>MQALRRGAAIPSRLLPRRDSWMSLAPFVAPNNAAAWRKLRDGAQEVQTVIERQSTPGKPQQIDWAKWESQIAHKDILNCLKTFYTNQVQILDRALGALETAKTPAPCEGAEKGWALFDAALSACAKSVEKSEELLSNGARALWVSCSNPPVWKVNTNEWLDSDQYWQAFVEKHHFYSQYQPGVVDPEAPQEVEAFKQAWHSRMGKFNDRSDTPMLYAYMNELPSWEYYDLHRSAFLEHMTYFLVRTGGDFRFFPEMPPWQWLAHMENLRFKLLSVAQSRRSQLQLANLERERALDFLPVDVEHHGEEYTQKFLQYETELFQACAARLMGHFMFLCDPFIPVQSAEALSAVTRVDNGKGKLFSLGDDVNALFYLPEQQRRDVERPTQAVQTLLGHLEATGRPFNPCYSELLHVHAEVLEERGEHWLTAPGECVSQAFLRRLRTDDPAYEVYCSYFKEMYERFAGAKEVSMEDGRKRLATIEKNAQEEAAAYGLALKTMGSAELAHKAREGAAKLEQLRKAQEKAAGKSAQTVQENKM[2x];>MTIHSCLARRAVSVAASGARAFASGLGARAVAVGALQSARLLHTSSLRAAGAKISPSEMSRLLEERIAGWKTQTSTEEVGRVVSVGDGIARLFGLEGVQAGELVEFQNGMTGMALNLETDNVGVVIFGDDRSVLEGDSVKRTGRIVDVPIGPGLLGRVVDALGNPIDGKGPIPAKERRRVELKAPGIIPRKSVHEPMMTGLKCVDALVPVGRGQRELIIGDRQTGKTAVAVDAIINQKEINDSTDDESKKLYCIYVAVGQKRSTVAQIVKALEQRDAMKYTTVVAATASEAAPLQFLAPYSGCAMGEWFRDSGRHCVIIYDDLSKQATAYRQMSLLLRRPPGREAYPGDVFYLHSRLLERAAKMGDKSGGGSLTALPVIETQAGDVSAYIPTNVISITDGQIFLETELFYKGIRPAINVGLSVSRVGSAAQVKAMKQVAGTMKLELAQYREVAAFAQFGSDLDASTRQLLTRGTALTELLKQRQYSPMKNSVQVCVLYCGVKGYLDPLDPKEISRFESLFIDYINANHQDILKTIETEKELSEKTEAKLRAAVDEFVAMNEFKKK[6x];>[2x]MNFSSSARWLAVRQSQTLGHTTRATVAAGRRVLAHSPAATEFTSFQSLHIGGDVCKLPLAVALGAAPSALGYGSAKHNQQRQYATLGSGWSFSKVQYTKYRITKPWTTDTTFDDIILSQPSKEDFAKFTKEAPLFLRFLKLVTDVEGRQEAFIQFAKRCENGLTVEKDVYVTKKELVDCLWKNGYTDTEINAFEIAFPADYKFHYPELAVLFDLTEEDCYKYCIRQRAATPEELVELKYTKPKNLVSSYGLCFLGVWFGLSNTVLSNAWFYSKTFPFGAVFYMLGSYFYRDIREKLWKEEKSLIHTAQENKNMGEESVYKQMKKYATDTKCLDYLSTFRTEVEDQIANYKVALVSQMRRQLTERLVEKLNGIQQAEKLIQGSLQDVMIREIVSSFKDLYKSRPELHDAAMQSAIQGLSGSDGAMDPVGAHFKASLQELAKVNLSTATADPMGTVVQRVAAVFQKREKEFLDTFTVKATEAQEIKTIVDKCHKGNTFDFHALSDEELRRLEQLYSTVNNRVGFETIHENSIKPVAPLSENSKGFVEFVNTQLEITKAKLRNARLTAFAHAFV;>[6x]MASPALQTCWRNLARLSGAQVRPSHFGAFSLGSRMSPFSSLLGARASPIATGRAGLRFLSSAAPNPGKKPASAAPPAGTNHGRITQVIGAVVDVHFDEQLPPILNSLEVQGHTNRLVLEVAQHLGENTVRTIAMDATEGLVRGQKVVDTGAPIQVPVGVETLGRIMNVIGEPVDECGPVPAKKTYSIHRAAPLFADQSTEPGLLQTGIKVVDLLAPYAKGGKIGLFGGAGVGKTVLIMELINNVANKHGGFSVFAGVGERTREGNDLYHEMMTTGVIKRKKLEDGKFDFTGSKAALVYGQMNEPPGARARVALTALSVAEYFRDEQGQDVLLFIDNIYRFTQAGSEVSALLGRIPSAVGYQPTLATDLGQLQERITTTKKGSITSVQAVYVPADDLTDPAPATTFAHLDATTVLSRQIAELGIYPAVDPLDSTSRMLAPEIVGQEHYDTARATQKLLQDYKSLQDIIAILGMDELSEEDKLVVSRARKIQRFLSQPFTVAEVFTGKPGRFVELPETIKSAQTILRGECDDLPEMAFYMCGGLEEVRSKAVKMAQEAASGK;>MGGGGGGALNKLFPGYKDKIWMKVPVQWRQQMIQHWNKSYEKQVYSESVALNRTFQARNQLVLDRLKPSGAYRLPAVDYKRQLSRGTLVEGADFYLPTAQEQQRLARHFEPYSEQEQEERRKFRFQSISVYLAVALGASFVHDYFYQRRPVAWCLEKEPPHPPSYPFWFKSLFHSHDIPSVRRGYEVYRKVCATCHSMEQLHFRHLVGEVLPEKRVKQIAAEYDVTDGPNDQGEMYTRPGILGDAFPSPYPNEEAARYANGGAYPPDLSLITAARHFGPDYLMALLGGYRDPPEGVELRPGLYWNVWFPGNAIAMPPPLMDEMIDYEDGTPCNISQMSKDVVNFLTWATEPTADERKLYGLKCVSAIAIGTVLMTLWWRFYWAMYATRRIDFGKLKYL[2x];>MSPVGRLFLGSKLPAQTWQSFRLQPALPQFAQKRFFSGGAAKPSWHVAREHRFGPTLPDHAYYGEHATYNYFVLFIRGMRPYLEKIFGDCASTIKNAAVAVYRPVNAFVVKHNPDLRLQFVAFASFIATHMAITKEFNDMYQRLVDITSLLELQAAQLHASEGFWDSESEQQEARLQRHAEHRNDLETTWEEALREATLARNFDVLVSYLNHGTSDGCGEHGACGHSGQNGIPPSVTWNFNAMPYGKENPDTKTFPIPDHEQPYRAFSLGFTANNLSGNWGDYIDRQDNKNALMRPARMMFTDVFIPTTK[2x];>MGEKQEEEGEEEKEGKGEGGGEGGREEEDEDGSAPVVSWLRIVEERECHEETDEAPETKIALPFSAQRSSRGFEARQVEVLVSANSAFLLSVLLASLFLSSSLPSFCPPRFLLSVLLALFKDKMAGDAPAAAAAPQQAGRTASASGVRTPGYLDLVGHSLKATSMDHGMQYSSIYWETSHRTYLPFWASLTQKFSWKIMDDQIRSFLRLPKPVTTEPFVFSSGSPYIRRYFGDADISVPVPLHAPAHFAFVPTGTVSPWEETGMETGPQGAAARGAAATAFRAVLESAWKCDIDEQIKEKLHSRAGAGAFHASGSTGGCPIPTDF[2x];>MALNRVPSRVLPFAVSGVYVHPRNACRLPAAAAVSSVPSSVSAFSSRTNFLSRSSSAVMSHPCAATARHFSFAIPPANAAALADPLPATPTPPPVFEAVSSASSGIASGTNALKNVEEVSTMERYEAAVYEESFKKPIVCLFFARFSLQSKVLLQPFLDFAASASNNATFFLIDCDRVPRAAYHARVENVPSLVVMKGDDAFRQTITDSVGVKTAGDLIQEARSALDQVLRLDQQEGGTKLQPGVSSYTHHIGVDNLNVYRKGWPVA[2x];>[2x]MQNGVFTRENADFLVKSGADSPSSQSLLLRTSPSPLSLPRRRFIFLRSASVDLSERSSLACLAPFFCLASGVCLRSAFSLPFFARRGRPCLFFIFIFFFRVSFTANFRGKRVKMAASTIPISQWPSLLYAPPSSPANPAVEALPEMQFDDLHYPRQMLLCRGAGYSLEQCNRMAQPDARVTPENPAEKLLKEEAVAAIACLSQREGGKDEQCRYYIERMYKLANKEKQPEPGTLSKASTLACKLLGIHRPEA;>[2x]MALPLLASRRLFSSFVFRGQPSTLSSNLSLVRIRGLHGGSLSPPSATLPRAVQLFSSRIAFSTAAAEDSGASQTLEGRYASALFRVAKKKNQLEKVYGDLESVRNALKDSSEFRLFVDSPAVSVQQKLDVLRQLVNRYKFDPLTGNLLTTLVENKRLPMLARVADAFDAMYRKEKGEVKCLVTSAKPLSAQQQKEIVAALQNRAGTQARLIIDYAVSPQIMGGLVVRLGEQVLDFSVATRLDRLQSQLLAPL;>MAETREGGQSGAASILGAEAFPELLSKVPLNPQMDEDKHFNKYKWGNEPIPVNRRTGSRMNSSIYDNRNHEAVRHPWSTDARTFHPNDNPEADRINTQYSNMVSDSFPEGGFSDAPRFSSNWERLLAYHHGLYSPEKFNSTTKTADEIRLAVNDFAAKVHADDPKNACKYLMIEEFKCLQSAQARIDPQGAATKCVKWFNEWRQCAWDQEKMVKGYNYIEDRRARKHKPYIGAPDLQYS[2x];>MFFSRLSLSALKAAPAREALPGLLSRQSFSSAGFSQFSSQKFFFSPSRNFSQSPLFQKHTPVHCNQRIASALVPTQQPAMTRQNPYAMQVGARYDAGVASLSAAIALMSVGGVAQGIGSLFAALVSGTARNPSIKEDLFTYTLIGMGFLEFLGIICVLMSAVLLYS[20x];>MPSSSSEDAQGGNRFECVSNSTSPRRKNATKDEAACLQPRRSAVSGPREDVLCIRTTPQPHVRRGKSGPGRRKRMRFGRERERRDKKRGEGERKRTRFPFLRLHIEGGNANSRRPLCFPSRHSLLRNHYGSLSMAFRKVSPPKAPMSVFEARSSFLDLEQCARAAGPQRWEAECQGVRQRALQAAADVMSRECGAYGDSFFQCYRHGFRLEACQGEKATMQLLRCQRMVADRLVPL[2x];>MGLSPAFAATAGCRLASPVANSSRFLSLLRLSRPRLNAAAPAAEAAKTLERNVPMKEILQPLWVVEPPNFLRQPVWKQFWEAQFANRSFFFFGNAWTSAAAFAFFIWWSRVFDPPPKERLDRYWLNSPKFRILSAFHNPGKRPGLKISLMTYEARYCYRGLDHPFTLNEMKDFLFKLREQYLVNKYEGIQFPFVFRQFNRVSTPGTLEVHTSPALQQQPHFHEEAAGHH[2x];>[2x]MAAGSRFPFCTAARLSSRGTLPRLGEATFFAGAESQRSAGAFAKTLQRPFLRAPSTQLFPVGNRLGVSSARALVANAMEPRRFFAAAASAKATHALQPTGTGSVAFTRPGQGSNAQFQTSLADKTRGLLGVGFLRPTKMASFAATFLLNFRFYFMYMARTTFQAVRPLLAFSVFGEVMKLVLATMSSGLFSFLFSFVLAFEVFYFFLQCYISYTFLTMFFTVLF;>[2x]MTALPPPPSANVAVSFTAAPAEPLSRGEVKAASLKLELQNIERELKDWWMSRKILRDRNIGLFNLLQHHNFAGLSVNNAKLSDSQRVMWTDLVQGKPDVEDKLSVDAREMKVDMYEKLFKQAADLENPCRMPGVAYLRCLRDTLTETQSARRSSCLNAFSSFDACRTGLLKQQSAAVENSLVRQNMADVRAKALFERRAVLLDLVEGK;>[2x]MNTFFLTPAAAAARRVAVSFFARSSASGFPQHRVALRPFPSQRPAERAHNLAKSQTLRSVKAHGRQSGKKEQSTESGGRRGFRAAVGAGTGCMLAASPMLFTDYDNTASPKSELIFMAGNALGYCTERFFENEYGQSIFMFALGLAYLAMLGHEGKIHGAVWRMKHLFATNFKMVGHPRYAYALPKNPLLQDAAPTKTGSTSAKK;>MSGDSVAPHQRAACEQLHSEYKQCLAKNGRTHFSACTDFHSKLRACENMLGTSYCIDEGINLMKCTKNPDPSFCAKEFVAMRECNRPQGPHLVLSSSPSSPPHYELRPEVKHLYNVDSTDLGSAVAPVRSKEQLDRVADSLKADLNLPGYGHIPYKWESLRPNPGA[2x];>MAFAGAAAPLGVKGRSVFAGMRSFIGQRLGRLYDSFYYSQSSTKYVMVFLFPAGIFYTRFRADTKLGYHVFINEEKLYPDYSQNYFDTKWTNGRKVYLDDETTVEQLKAQIYGGKAAPENVKVACRGRVFEDADNVAMAVRAFCKRDPRLLLFQDNL[2x];>[2x]MSPPTASASVASSGSSPHMDRLLGDLKLLAAYDSAAGWQEPKAMESAFQSLSWDDADVLKALPQYLNCRGEQKRRVDFAYAALCPRPVDEKDPKQTLMSLWMKARLFSYDQKHPFVLSPFAATDKSTSAGAMTAEKPF;>[2x]MVRNQRYPASPVQEIFLPEPVPFVQFDQTAPSPNSPPAPLPSPSLSQCEEQKDRYRDISSMFHRGVAGAEQVREAYNSMAKCFRRVSVAEVLESDPAFRQARNFTMDLKQAEDDQRYKQLQYGRVPSILTKYHL;>[2x]MLNFIPKRCPSVSLLFGKRPVQRIEVGQARHQLEIPVETIEKIYEGVDSRLEYHNKDYNAMKWKDFMKLKLDAYHLLEASQSETAAKSALSDLNWFSDLADIYSGQQTMAEMDVALKAQGEQKLSYPIQGKNIK;>MSWATRLLRMSSPRLGLLPLGRSVKLGGAKERVSFSQFFDSEYFWTKANVGPFFLFLFTSPFWYQGIKTVYASCRYRKLNEREIISDRYTWLHERMLEDEVERVLLEQVPAGGFDKTRPGLLLGPSTL[2x];>MPAPAASGAAAVLSKDIARSFRWMQAFAAVKGKPTAGSCAAGTAVVNPEDPTKVTLKGRYTNFSLQHIWEKYDYLQTHLLLRECMLSQVAKNPRLLDPEINAGLTPTVFMRVPPETQDPETQAKAAPQKGQAN[2x];>MATPPLQDGAPTNGGAATKPSCGARLQNFARMAIKGPSVPHSILFGVGAGCCAYAGYYLYRAMRLTFFDTESVALQSRLRYAEKQKLFHQELDRELAAGHIASLVAEYDPVATRLPFQPMQDRYRV[2x];>MGFHFQQYIAMAGRAINPVQWTRAWRRMEGKSATEVYRDALAWTNNQFAQISRASQYRAWWWQNPLGMGLVLYGTYKAWHMIYMVRKQKKTAQLVAAAYGQGGQWLNPVPR[2x];>MPFMWRQRAYCAPVPSAFASQQPNGLGGEAGVRKPLLRSNSESLSVFSQIPDGLLGHTTSVTMGNSDIFFLPKPSNLLKIALPAFVFMPNLTIFTRAFPFYAHTSA[2x];>MSTSPGLAFANLTLLLDVPQLPAIWAVNAWRELNGLFTEMKTLAGTSDLLYPSNRYNPQNEKTNRMGRPRKYNHGEWMFGNSY[2x];>MFARAFSRFASLAAPAPQRGWNAFVLPSRHFATAAGGANPFKNQLLLTLSSPSEAIYVRTPVRSVTVPGSEGAMTMTNGHSQTVARLKAGEIIVRKGETGDEVERFFLSDGFVLFKSPEDDSGCCTAEVLGVEVVPVSMLDKESAATALQELLQQGAGATDEWTKARTLLGQELLSSVIRAAP[2x];>[2x]MWRSSGVSFTRYASEMAALLRQCLKEPYRTQAMQRNQIHLKETVYQQGQVLTRETFNDIKKAFEAAAKHAGEK;>MAGLASLSSVGALRGMRLVPAAHLLPLHSAFGQQTRNFGAGDLKIVAARMKSVKSIQKITKAMKMVAASKLRMDQRRLENGLPFATPVQKLVQRIPVDPKEKGTLAVLALSSDKGLCGGVNSFVAKQARIVIKENEMAGNAVQVYGVGDKIRSALQRTFGDRFKRIMTEVTRFPWNFGQACIIADRLMQDNPARLMVIYNHFKSAVAYDTLTLNVLTPTQAAQSAKEQLNTFEFEPEKTDVWKDLQDFYYACTVFGCMLDNIASEQSARMSAMDNASTNAGEMISSLTLRYNRARQAKITTELVEIISGANALE[2x];>MSSPCCVAIRRVARTTLESGRRQVDSKSTDVSPFFTGTQQMSLPSAGMVTKIRNFSSVKFMDQKRSGEETVYFKKEDEALLRNLLANHPEYDPKYSVDHMNAEVGSIARDITLACQKHGMKDPSAAFMKDLISIFGAHGYAKNSK[2x]

F-type ATP synthases are energy-converting membrane protein complexes that synthesize adenosine triphosphate (ATP) from ADP and inorganic phosphate. These universal enzymes function by using the energy stored in an electrochemical potential across the bioenergetic membrane by rotary catalysis. In mitochondria, F1Fo ATP synthase resides in the crista membrane where it is known to form dimers, which can further assemble into rows critical for inducing the membrane curvature and maintaining membrane potential and morphology. Here, we investigate the mechanism for the generation of the unique cristae in the Apicomplexa, using a combination of single-particle cryo-EM, cryo-ET and subtomogram averaging.

We then performed solubilisation with n-dodecyl-β-D-maltoside (β–DDM) that resulted in dissociation of the hexamers into dimers. Refinement into a 2.9-Å resolution consensus map allowed model construction of the entire ATP synthase dimer. The 1.85-MDa complex consists of 32 different subunits, of which only 15 are canonical with structural equivalents in other phyla. The apicomplexan-conserved subunits and extensions of the canonical subunits constitute a membrane-embedded Fo subcomplex, which ties the two F1/c-ring subcomplexes together at the angle of 19°. This is in stark contrast to ~100° found in the yeast and mammalian ATP synthase dimers, suggesting the narrow-angle parasite dimer induces substantially less membrane curvature. The structure of the T. gondii ATP synthase reveals that the unusual architecture of the dimer is generated by the peripheral stalks that are laterally offset, extending away from the central dimer axis. This architecture does not allow the formation of the conventional dimerization interface of type-I ATP synthases found in animals and yeast, in which peripheral stalks extend along the dimer long axis. We therefore examined the dimerization interface, which is formed by the apicomplexan subunits and extensions of the canonical Fo subunits. Those elements involve eleven proteins from each monomer that contribute more than 7000 Å2 of buried surface area, making the interface substantially larger than in mammalian, yeast and algal ATP synthase structures. The inhibitor protein of ATPase activity IF1 is bound to subunit-b, contributing to the Fo dimer interface with its C-terminal helix extending from F1 to interact with subunit-b’ of the neighbouring monomer.>SLEPVKNIIHNSIDDLIDEFNLLENVSDELYELKKLNNLDEKYLISFEDISKNNSTYSVRFINKSNGESVYVETEKEIFSKYSEHITKEISTIKNSIITDVNGNLLDNIQLDHTSQVNTLNAAFFIQSLIDYSSNKDVLNDLSTSVKVQLYAQLFSTGLNTIYDSIQLVNLISNAVNDTINVLPTITEGIPIVSTILDGINLGAAIKELLDEHDPLLKKELEAKVGVLAINMSLSIAATVASIVGIGAEVTIFLLPIAGISAGIPSLVNNELILHDKATSVVNYFNHLSESKKYGPLKTEDDKILVPIDDLVISEIDFNNNSIKLGTCNILAMEGGSGHTVTGNIDHFFSSPSISSHIPSLSIYSAIGIETENLDFSKKIMMLPNAPSRVFWWETGAVPGLRSLENDGTRLLDSIRDLYPGKFYWRFYAFFDYAITTLKPVYEDTNIKIKLDKDTRNFIMPTITTNEIRNKLSYSFDGAGGTYSLLLSSYPISTNINLSKDDLWIFNIDNEVREISIENGTIKKGKLIKDVLSKIDINKNKLIIGNQTIDFSGDIDNKDRYIFLTCELDDKISLIIEINLVAKSYSLLLSGDKNYLISNLSNTIEKINTLGLDSKNIAYNYTDESNNKYFGAISKTSQKSIIHYKKDSKNILEFYNDSTLEFNSKDFIAEDINVFMKDDINTITGKYYVDNNTDKSIDFSISLVSKNQVKVNGLYLNESVYSSYLDFVKNSDGHHNTSNFMNLFLDNISFWKLFGFENINFVIDKYFTLVGKTNLGYVEFICDNNKNIDIYFGEWKTSSSKSTIFSGNGRNVVVEPIYNPDTGEDISTSLDFSYEPLYGIDRYINKVLIAPDLYTSLININTNYYSNEYYPEIIVLNPNTFHKKVNINLDSSSFEYKWSTEGSDFILVRYLEESNKKILQKIRIKGILSNTQSFNKMSIDFKDIKKLSLGYIMSNFKSFNSENELDRDHLGFKIIDNKTYYYDEDSKLVKGLININNSLFYFDPIEFNLVTGWQTINGKKYYFDINTGAALTSYKIINGKHFYFNNDGVMQLGVFKGPDGFEYFAPANTQNNNIEGQAIVYQSKFLTLNGKKYYFDNNSKAVTGWRIINNEKYYFNPNNAIAAVGLQVIDNNKYYFNPDTAIISKGWQTVNGSRYYFDTDTAIAFNGYKTIDGKHFYFDSDCVVKIGVFSTSNGFEYFAPANTYNNNIEGQAIVYQSKFLTLNGKKYYFDNNSKAVTGLQTIDSKKYYFNTNTAEAATGWQTIDGKKYYFNTNTAEAATGWQTIDGKKYYFNTNTAIASTGYTIINGKHFYFNTDGIMQIGVFKGPNGFEYFAPANTDANNIEGQAILYQNEFLTLNGKKYYFGSDSKAVTGWRIINNKKYYFNPNNAIAAIHLCTINNDKYYFSYDGILQNGYITIERNNFYFDANNESKMVTGVFKGPNGFEYFAPANTHNNNIEGQAIVYQNKFLTLNGKKYYFDNDSKAVTGWQTIDGKKYYFNLNTAEAATGWQTIDGKKYYFNLNTAEAATGWQTIDGKKYYFNTNTFIASTGYTSINGKHFYFNTDGIMQIGVFKGPNGFEYFAP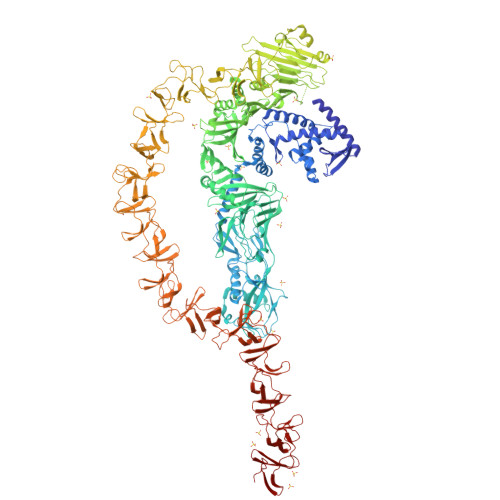ANTDANNIEGQAILYQNKFLTLNGKKYYFGSDSKAVTGLRTIDGKKYYFNTNTAVAVT[2x]{4-[2-ACETYLAMINO-2-(1-BIPHENYL-4-YLMETHYL-2-OXO-AZEPAN-3-YLCARBAMOYL)-ETHYL]-2-PHOSPHONO-PHENOXY}-ACETIC 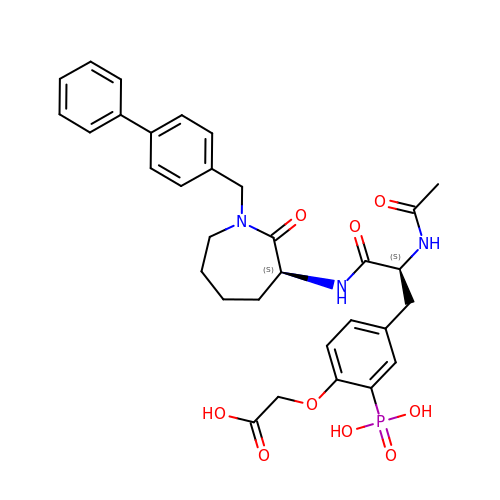ACID | C32 H36 N3 O9 P | MWEWSHNGVWABKG-SVBPBHIXSA-N>SYYIDADLLREIKQHLKQQQEGLSHLISIIKDDLE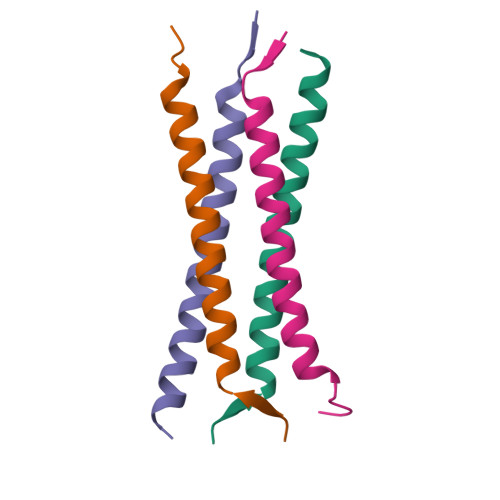DIKLV[4x]>[4x]MDKLPPSMRKRLYSLPQQVGAKAWIMDEEEDAEEEGAGGRQDPRRRSIRLRPLPSPSPSPSAAAAAAGGAESRGAALGGAADGEGPARGAAKSSTNGDCRRFRGSLASLGSRGGGGGGGSTGGGSHGHLHDSAEERRLIAEGDASPGEDRTPPGLAAEPERPGAPAPPAASPPQVPSSCGEQRPADAAVKVEGGAAAGDQILPEAEARLGQAGFMQRQFGAMLQPGVNKFSLRMFGSQKAVEREQERVKSAGFWIIHPYS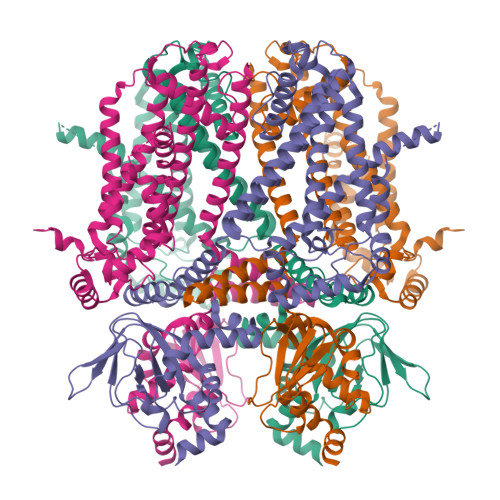DFRFYWDLTMLLLMVGNLIIIPVGITFFKDENTTPWIVFNVVSDTFFLIDLVLNFRTGIVVEDNTDIILDPRRIKMKYLKSWFVVDFVSSIPVDYIFLIVETRIDSEVYKTARALRIVRFTKILSLLRLLRLSRLIRYIHQWEEIFHMTYDLASAVVRIVNLIGMMLLLCHWDGCLQFLVPMLQDFPDDCWVSLNNMVNNSWGKQYSYALFKAMSHMLCIGYGRQAPMGMSDVWLTMLSMIVGATCYAMFIGHATALIQSLDSSRRQYQEKYKQVEQYMSFHKLPPDTRQRIHDYYEHRYQGKMFDEESILGELSEPLREEIINFNCRKLVASMPLFANADPNFVTSMLTKLRFEVFQPGDYIIREGTIGKKMYFIQHGVVSVLTKGNKETKLADGSYFGEICLLTRGRRTASVRADTYCRLYSLSVDNFNEVLEEYPMMRRAFETVALDRLDRIGKKNSIHKVQHDLSSGVSNYQENAIVQRIVQHDREMAHCARRAQATTPVAPAIWTPLIQAPLQAAAQDLKLISASQPALPQDGAQTLRRASPHSSSGESVAALPPAGGPFPRAPGRPPGAGPGQHVTLTLPRKASSGSLPPPLSLFGPRAAPRLTAAPQREPGAKSEPVRSKLP>MDIKINDITLGNNSPFVLFGGINVLESLDSTLQTCAHYVEVTRKLGIPYIFKASFDAANRSSIHSYRGVGLEEGLKIFEKVKAEFGIPVITDVHEPHQCQPVAEVCDVIQLPAFLARQTDLVVAMAKTGNVVNIKKPQFLSPSQMKNIV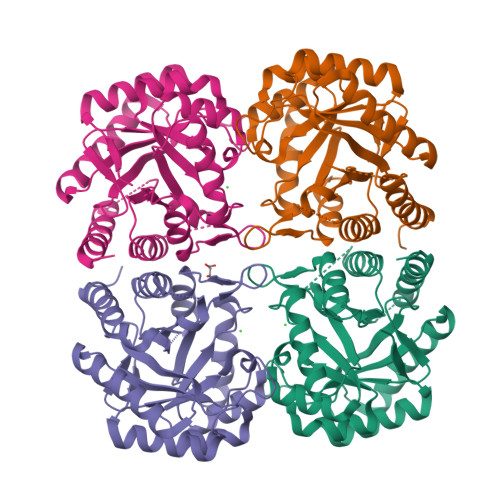EKFHEAGNGKLILCERGSSFGYDNLVVDMLGFGVMKQTCGNLPVIFDVTHSLQTRDAGSAASGGRRAQALDLALAGMATRLAGLFLESHPDPKLAKCDGPSALPLHLLEDFLIRIKALDDLIKSQPILTIE[4x]Anti-phage systems of the BREX (BacteRiophage EXclusion) superfamily rely on site-specific epigenetic DNA methylation to discriminate between the host and invading DNA. We demonstrate that in Type I BREX systems, defense and methylation require BREX site DNA binding by the BrxX (PglX) methyltransferase employing S-adenosyl methionine as a cofactor. We show that BrxX contains MTD and TRD homologous to those of Type IIL R-M enzymes, and, in addition, contains NTD, CTD, and insertion loop in the MTD specific to BrxX proteins. We show that BrxX alone does not methylate DNA, and BREX activity requires an assembly of a supramolecular BrxBCXZ immune complex.

Ocr inhibits BREX defense by binding BrxX in vivo. 57% of the extracted particles yielded a 2.8 Å global resolution map (BrxX:Ocr) corresponding to a BrxX2:Ocr2 complex where two individual BrxX monomers interact with a dimer of Ocr via their TRDs and CTDs. The two BrxX monomers are oriented at an angle of 125° relative to each other; however, the complex displays imperfect symmetry due to the local flexibility of the individual components resulting in varied local resolution. We resolved one monomer to ~2.8 Å clearly defining all structural features except for a flexible loop between residues 395 and 420. The map resolution for the second BrxX monomer stretched from ~3.4 Å around the core of the particle to ~4–6 Å at the periphery; hence, we rigid-body fitted the first monomer model into the density of the second monomer (see “Methods”). Ocr is highly negatively charged, and its interaction with BrxX is largely driven by electrostatic contacts with the positively charged groove on the lower half of the BrxX monomer. To form direct contacts, Ocr utilizes two pairs of tyrosine and glutamic acid residues that form hydrogen bonds with four residues of BrxX TRD: T821, N823, T768, and the main-chain carbonyl of G721. Three out of four of these TRD residues are also directly involved in DNA recognition or binding: N823 directly interacts with the A4 in the target strand of the recognition site, while the main-chain amide of G721 interacts with the phosphate backbone of T5′ base in the non-target strand. Ocr is additionally stabilized by the BrxX CTD via a salt bridge between Ocr E67 and BrxX R1145; the latter residue also interacts with the DNA away from the recognition site. The DNA mimic protein Ocr exploits this non-specific DNA recognition property to sequester BrxX (Stage VI).

>[2x]MNTNNIKKYAPQARNDFRDAVIQKLTTLGIAADKKGNLQIAEAETIGETVRYGQFDYPLSTLPRRERLVKRAREQGFEVLVEHCAYTWFNRLCAIRYMELHGYLDHGFRMLSHPETPTAFEVLDHVPEVAEALLPESKAQLVEMKLSGNQDEALYRELLLGQCHALHHAMPFLFEAVDDEAELLLPDNLTRTDSILRGLVDDIPEEDWEQVEVIGWLYQFYISEKKDAVIGKVVKSEDIPAATQLFTPNWIVQYLVQNSVGRQWLQTYPDSPLKDKMEYYIEPAEQTPEVQAQLAAITPASIEPESIKVLDPACGSGHILTEAYNVLKAIYEERGYRTRDIPQLILENNIFGLDIDDRAAQLSGFAMLMLARQDDRRILGRGVRLNIVSLQESKLDIAEVWTKLNFHQHMQRGSMGDMFTQGTALANTDSAEYKLLMRTLALFTSAKTLGSLIQVPQEDEAALKAFLERLYRLAVEGDIQQKEAAAELIPYIQQAWILAQRYDAVVANPPYMGGKGMNGDLKEFAKKQFPDSKSDLFAMFMQHAFSLLKENGFNAQVNMQSWMFLSSYEALRGWLLDNKTFITMAHLGARAFGQISGEVVQTTAWVIKNNHSGFYKPVFFRLVDDNEEHKKNNLLNRMNCFKNTLQNDFKKIPGSPIAYWATLAFINSFLKLPALGTRAVKGLDTNGSIDVFLRRWPEVSINSFDALGKGNSKWFPIAKGGELRKWFGNHEYIINYENDGIELRKNKANLRNKDMYFQEGGTWTVVSTTGFSMRYMPKGFLFDQGGSAVFCENNDELSIYNILACMNSKYINYSASLICPTLNFTTGDVRKFPVIKNNHLEDLAKKAIEISKADWNQFETSWEFSKNKLIEHKGNVAYSYASYCNFQDKLYEQLVNIEKNINNIIEEILGFKIETTENSELITLNSNKIYRYGQSETNDTFLNRHRSDTISELISYSVGCQMGRYSLDREGLVYAHEGNKGFAELAAEGAYKTFPADNDGILPLMDDEWFEDDVTSRVKEFVRTVWGEEHLQENLEFIAESLCLYAIKPKKGESALETIRRYLSTQFWKDHMKMYKKRPIYWLFSSGKEKAFECLVYLHRYNDATLSRMRTEYVVPLLARYQANIDRLNDQLDEASGGEATRLKRERDSLIKKFSELRSYDDRLRHYADMRISIDLDDGVKVNYGKFGDLLADVKAITGNAPEAI;>MAMSNMTYNNVFDHAYEMLKENIRYDDIRDTDDLHDAIHMAADNAVPHYYADIFSVMASEGIDLEFEDSGLMPDTKDVIRILQARIYEQLTIDLWEDAEDLLNEYLEEVEEYEEDEE[2x]> LTAKKRPSVVYLHNAECTGCSESLLRTVDPYVDELILDVISMDYHETLMAGAGHAVEEALHEAIKGDFVCVIEGGIPMGDGGYWGKVGRRNMYDICAEVAPKAKAVIA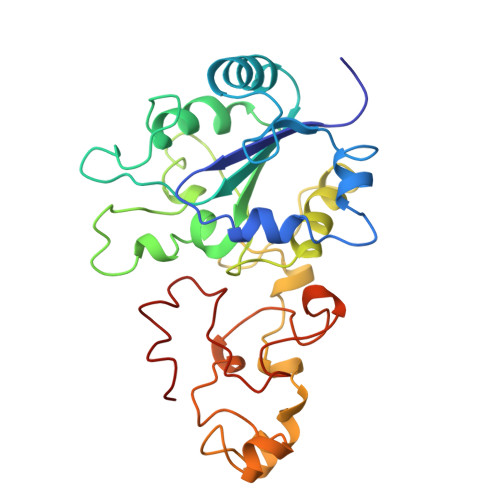IGTCATYGGVQAAKPNPTGTVGVNEALGKLGVKAINIAGCPPNPMNFVGTVVHLLTKGMPELDKQGRPVMFFGETVHDNCPRLKHFEAGEFATSFGSPEAKKGYCLYELGCKGPDTYNNCPKQLFNQVNWPVQAGHPCIACSEPNFWDLYSPFYSA>GPDSMRQLPYHADKLSWDEKHRVNEEQIYCYCGKPGKFDHNMLQCCKCRNWFHTQCMQNFKKKLLRGDMFFVFCCTVCNNGIEFVRRMQIEWVDVLHIALYNLRKHQHQKYHHLLNDIWPFILEQRHQLPICEKWRTLPETALMERLKQTLKDYSDRFVCGREFKRAPAFYALRHSGPPHIPKVFLEPHEELSDELLEKRFKLML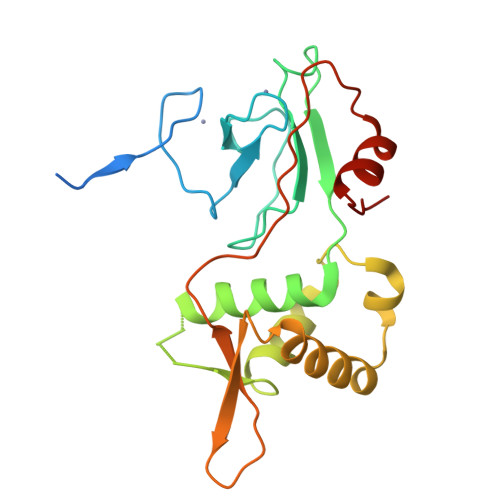MPEE[6x]>FEGDLKWHHHNITYWIQNYSEDLPRAVIDDAFARAFALWSAVTPLTFTRVYSRDADIVIQFGVAEHGDGYPFDGKDGLLAHAFPPGPGIQGDAHFDDDELWSLGKGQGYSLFLVAAHQFGHALGLDHSSVPEA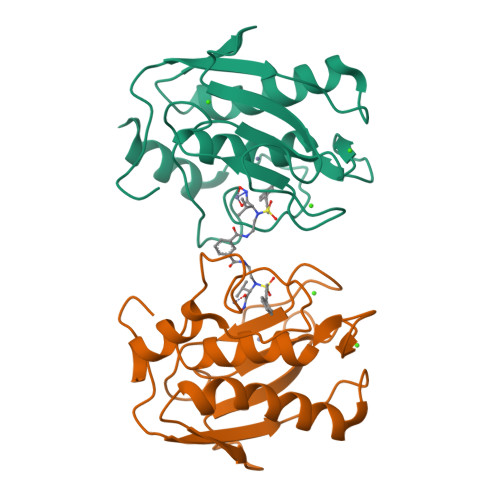LMYPMYRFTEGPPLHKDDVNGIRHLYG[4x]>[6x]MSLQLLRNTRIFVSTVKTGHNKTNTQEILVQDDISWGQDSNSTDITVNEAGPRPTRGSKRFNDSLNAAEWSFSTYILPYKDKNTSKQIVPDYMLWHALSSGRAINLEGTTGAHNNATNFMVNFKDNSYHELAMLHIYILTDKTWSYIDSCQINQAEVNVDIEDIGRVTWSGNGNQLIPLDEQPFDPDQIGIDDETYMTIQGSYIKNKLTILKIKDMDTNKSYDIPITGGTFTINNNITYLTPNVMSRVTIPIGSFTGAFELTGSLTAYLNDKSLGSMELYKDLIKTLKVVNRFEIALVLGGEYDDERPAAILVAKQAHVNIPTIETDDVLGTSVEFKAIPSDLDAGDEGYLGFSSKYTRTTINNLIVNGDGATDAVTAITVKSAGNVTTLNRSATLQMSVEVTPSSARNKEVTWAITAGDAATINATGLLRADASKTGAVTVEATAKDGSGVKGTKVITVTAGG;>MFYSLMRESKIVIEYDGRGYHFDALSNYDASTSFQEFKTLRRTIHNRTNYADSIINAQDPSSISLAINFSTTLIESNFFDWMGFTREGNSLFLPRNTPNIEPIMFNMYIINHNNSCIYFENCYVSTVDFSLDKSIPILNVGIESGKFSEVSTFRDGYTITQGEVLPYSAPAVYTNSSPLPALISASMSFQQQCSWREDRNIFDINKIYTNKRAYVNEMNASATLAFYYVKRLVGDKFLNLDPETRTPLIIKNKYVSITFPLARISKRLNFSDLYQVEY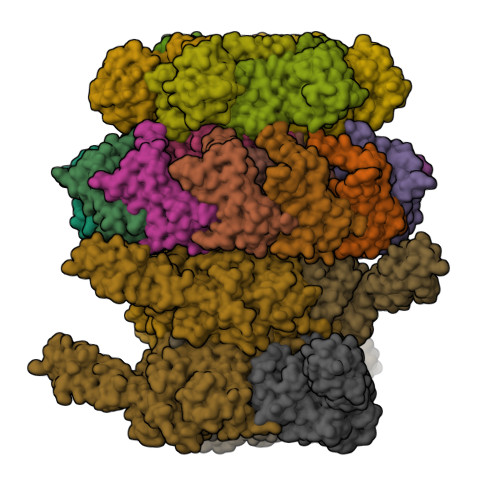DVIPTADSDPVEINFFGERK[3x];>MSTENRVIDLVVDENVPYGLLMQFMDVDDSVYPSTSKPVDLTDFSLRGSIKSSLEDGAETVASFTTAIVDAAQGVASISLPVSAVTTIASKASKERDRYNPRQRLAGYYDVIITRTAVGSAASSFRIMEGKVYISDGVTQ[12x];>[6x]MRLPDPYTNPEYPGLGFESVNLVDNDPMIRDELPNGKVKEVKISAQYWGINISYPELFPDEYAFLDSRLLEYKRTGDYLDVLLPQYEAFRVRGDTKSVTIPAGQKGSQIILNTNGTLTGQPKAGDLFKLSTHPKVYKITNFSSSGNVWNISLYPDLFITTTGSEKPVFNGILFRTKLMNGDSFGSTLNNNGTYSGISLSLRESL> VIGGDECNINEHRFLALVYANGSLCGGTLINQEWVLTARHCDRGNMRIYLGMHNLKVLNKDALRRFPKEKYFCLNTRNDTIWDKDIMLIRLNRPVRNSAHIAPLSLPSNPPSVGSVCRIMGWGTITSPNATLPDVPHCAN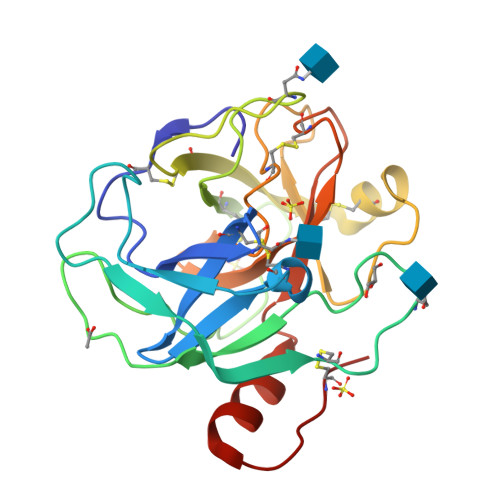INILDYAVCQAAYKGLAATTLCAGILEGGKDTCKGDSGGPLICNGQFQGILSVGGNPCAQPRKPGIYTKVFDYTDWIQSIISGNTDATCPP> NSYNTTNRHNLESLYKHDSNLIEADSIK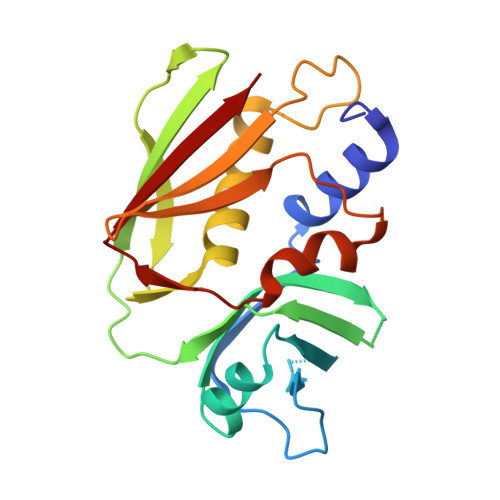NSPDIVTSHMLKYSVKDKNLSVFFEKDWISQEFKDKEVDIYALSAQEVCECPGKRYEAFGGITLTNSEKKEIKVPVNVWDKSKQQPPMFITVNKPKVTAQEVDIKVRKLLIKKYDIYNNREQKYSKGTVTLDLNSGKDIVFDLYYFGNGDFNSMLKIYSNNERIDSTQFHVDVSIS>[4x]MSQSPAFGPRRGSSPRGAAGAAARRNESQDYLLMDSELGEDGCPQAPLPCYGYYPCFRGSDNRLAHRRQTVLREKGRRLANRGPAYMFSDRSTSLSIEEERFLDAAEYGNIPVVRKMLEECHSLNVNCVDYMGQNALQLAVANEHLEITELLLKKENLSRVGDALLLAISKGYVRIVEAILSHPAFAEGKRLATSPSQSELQQDDFYAYDEDGTRFSHDVTPIILAAHCQEYEIVHTLLRKGARIERPHDYFCKCNDCNQKQKHDSFSHSRSRINAYKGLASPAYLSLSSEDPVMTALELSNELAVLANIEKEFKNDYKKLSMQCKDFVVGLLDLCRNTEEVEAILNGDVETLQSGDHGRPNLSRLKLAIKYEVKKFVAHPNCQQQLL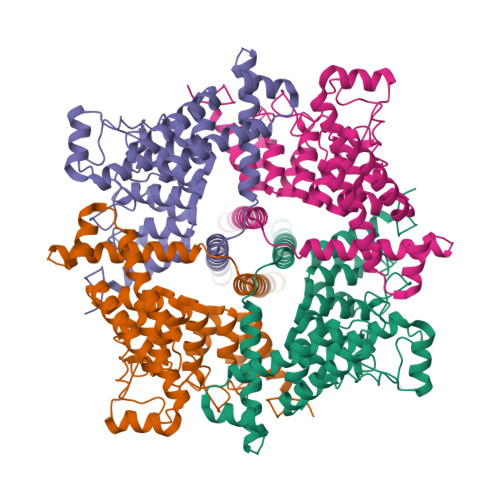SIWYENLSGLRQQTMAVKFLVVLAVAIGLPFLALIYWFAPCSKMGKIMRGPFMKFVAHAASFTIFLGLLVMNAADRFEGTKLLPNETSTDNAKQLFRMKTSCFSWMEMLIISWVIGMIWAECKEIWTQGPKEYLFELWNMLDFGMLAIFAASFIARFMAFWHASKAQSIIDANDTLKDLTKVTLGDNVKYYNLARIKWDPSDPQIISEGLYAIAVVLSFSRIAYILPANESFGPLQISLGRTVKDIFKFMVIFIMVFVAFMIGMFNLYSYYIGAKQNEAFTTVEESFKTLFWAIFGLSEVKSVVINYNHKFIENIGYVLYGVYNVTMVIVLLNMLIAMINSSFQEIEDDADVEWKFARAKLWFSYFEEGRTLPVPFNLVPSPKSLFYLLLKLKKWISELFQGHKKGFQEDAEMNKINEEKKLGILGSHEDLSKLSLDKKQVGHNKQPSIRSSEDFHLNSFNNPPRQYQKIMKRLIKRYVLQAQIDKESDEVNEGELKEIKQDISSLRYELLEEKSQNTEDLAELIRELGEKLSMEPNQEETNRAENLYFQSHHHHHHHHHHDYKDDDDK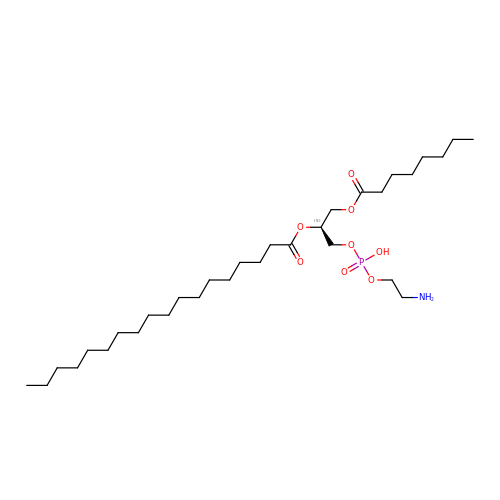[(2~{S})-1-[2-azanylethoxy(oxidanyl)phosphoryl]oxy-3-octanoyloxy-propan-2-yl] octadecanoate | C31 H62 N O8 P | UXEZQBUDEBPDGU-LJAQVGFWSA-N>RDRMVMGKIKRIEAGLPLTTAKGRTFGYDVIDTKLYINEEEAKQLRLIYDIFEEEQSITFLQKRLKKLGFKVRTYNRYNNWLTNDLYCGYVSYKDKVHVKGIHEPIISEEQFYRVQEIFSRMGKNPNMNKESASLLNNLVVCSKCGLGFVHRRKDTVSRGKKYHYRYYSCKTYKHTHELEKCGNKIWRADKLEELIIDRVNNYSFASRNIDKEDELDSLNEKLKIEHAKKKRLFDLYINGSYEVSELDSMMNDIDAQINYYEAQIEANEELKKNKKIQENLADLATVDFNSLEFREKQLYLKSLINKIYIDGEQVTIEWL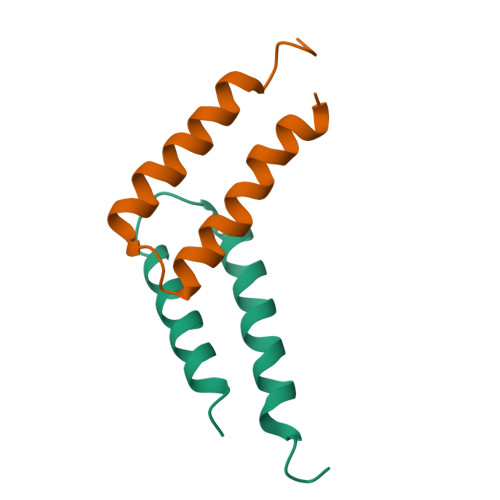LEHHHHHH[8x]6-chloro-2,3-dihydro-1H-isoindol-1-one | C8 H6 Cl N O | 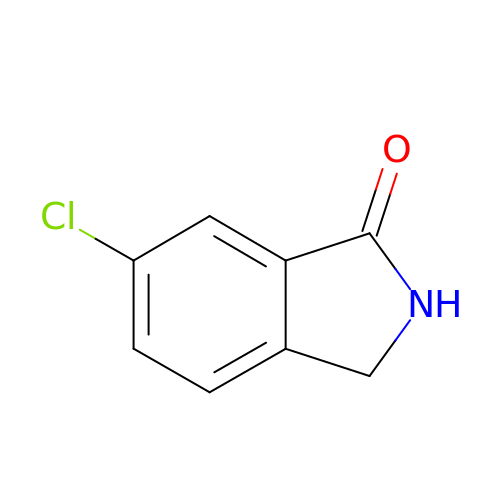VCEOKEOSVQLRNW-UHFFFAOYSA-N> MSEFRIHHDVNELLSLLRVHGGDGAEVYIDLLQKNRTPYVTTTVSAHSAKVKIAEFSRTPEDFLKKYDELKSKNTRNLDPLVYLLSKLMEDRETLQYLQQNAKERAELAASAAASSTASFGASATAS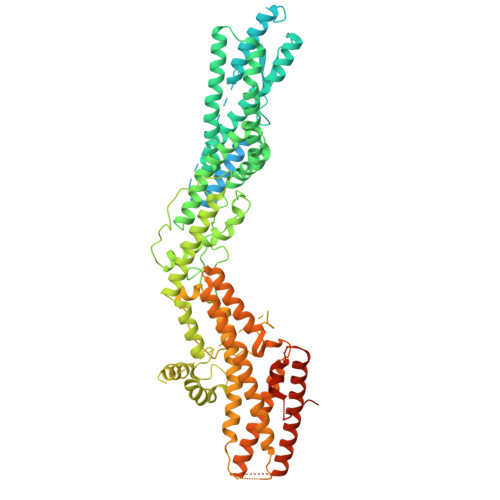KISMQELEELRKQLGSVATGPTWQQSLELTRKMLRDKQSKKNSGQRLPVLPAWVYERPALLGDFLPGTGGSADTAVPIGSLPLASQEAAVVEDLLYVLVGVDGRYISAQPLTGRQGRTFLVDPNLDLSIRELVSRILPVAASYSTVTRFIEEKSSFEYGQVNHALAAAMRTLVKEYLVLVTQLEQLQRQGLLSLQKLWFYIQPAMRSLDILASLATSVDKGECIGGATLSLLHDRSFSYTGDSQAQELCLHLTKAASTPYFEILEKWIYRGIIDDPYSEFMVEEHELRKEKIQEDYNDKYWDQRYTVVQRQIPSFLQKMAGKVLSTGKYLNVVRECGHDVTCPVAKEVVYTLKERAYVEQIEKAFSYASKVLLDFLMGEKELLAHLRSIKRYFLMDQGDFFVHFMDLTEEELKKPVDDITPTRLEALLELALRMSTANTDPFKDDLKIDLMPHDLITQLLRVLAIETQQEKAMVHADPTELTLSGLEAFSFDYVVTWPLSLIINRKALTRYQMLFRHMFYCKHVERQLCSVWISNKAAKRFSLHSAKWFAGAFTLRQRMLNFVQNIQSYMMFEVMEPTWHVLEQNLRSASNIDDVLGHHASFLDNCLKDCMLTNPELLRVFSKLMSVCVMFTNCLQRFTQSMKLDSELGHPALEPGAMLGPPTEAERAEERARKELARKCLAEHVDAPQLASSFEATITKFDKNFSAHLLDLLARLSIYSTSDCEHGMASVISRLDFNGFYTERLERLSAERSQKAAPPVPGPRGPPALVPRVAVTAQ> GAMDPMICLGLEGTAEKTGVGIVTSDGEVLFNKTIMYKPPKQGINPREAADHHAETFPKLIKEAFEVVDKNEIDLIAFSQGPGLGPSLRVTATVARTLSLTLKKPIIGVNHCIAHIEIGKLTTEAEDPLTLYVSGGNTQVIAYVSKKYRVFGETLDIAVGNCLDQFARYVNLPHPGGPYIEELARKGKKLVDLPYTVKGMDIAFSGLLTAAMRAYDAGERLEDICYSLQEYAFSMLTEITERALAHTNKGEVMLVGGVAANNRLREMLKAMCEGQNVD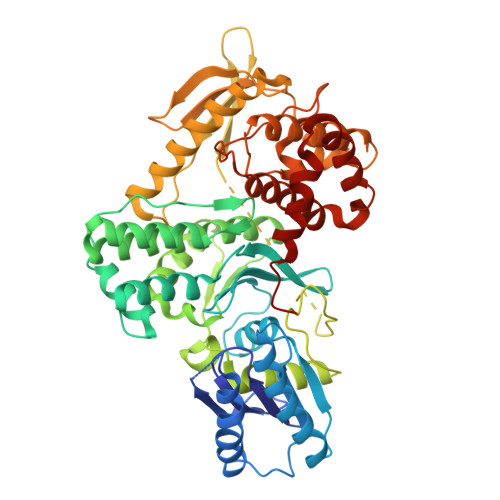FYVPPKEFCGDNGAMIAWLGLLMHKNGRWMSLDETKIIPNYRTDMVEVNWIKEIKGKKRKIPEHLIGKGAEADIKRDSYLDFDVIIKERVKKGYRDERLDENIRKSRTAREARYLALVKDFGIPAPYIFDVDLDNKRIMMSYINGKLAKDVIEDNLDIAYKIGEIVGKLHKNDVIHNDLTTSNFIFDKDLYIIDFGLGKISNLDEDKAVDLIVFKKAVLSTHHEKFDEIWERFLEGYKSVYDRWEIILELMKDVERRARYVE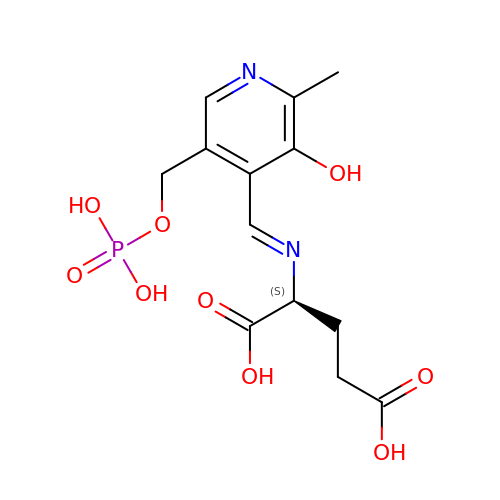(E)-N-({3-hydroxy-2-methyl-5-[(phosphonooxy)methyl]pyridin-4-yl}methylidene)-L-glutamic acid | C13 H17 N2 O9 P | ZZRWFCMLYWHYGX-XSFFOXFNSA-N>AECSVDIQGNDQMQFNTNAITVDKSCKQFTVNLSHPGNLPKNVMGHNWVLSTAADMQGVVTDGMASGLDKDYLKPDDSR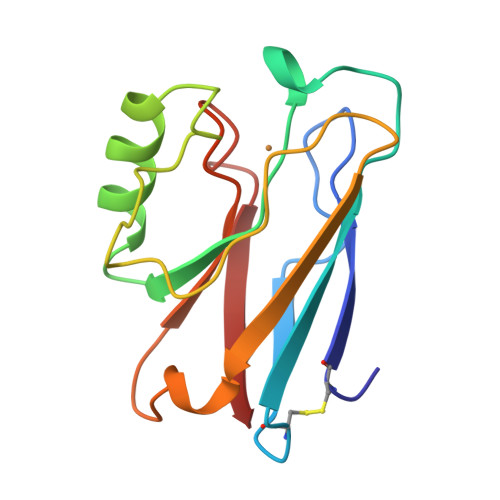VIAHTKLIGSGEKDSVTFDVSKLKEGEQYMSFCTFPGHSALMKGTLTLK[12x]> GMSRFWRSFTYFEWRPTPAIHRQLQKIICKYKETFMKQEYTNPYQLVDFDPLFISHLGAPKPLHVSLTRSLLFETEEQRHVFIQ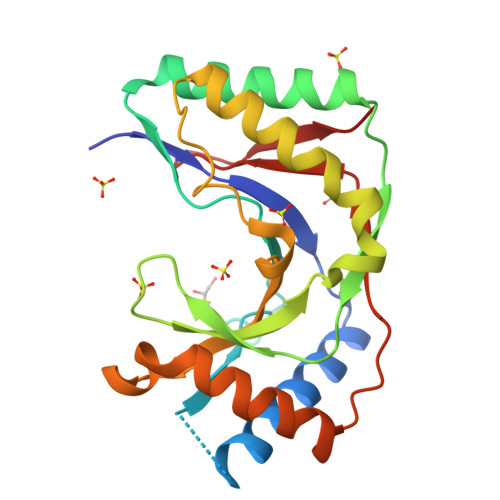EMRNGLRNNEITPFKLQICSYPKLYISERANTLYLGLPVSECPNKAQISPFKTIIAEALQKSGISNYQDLIVSRQNLHVSIAIASNPSKATLKRYQQLNETMGALLLLNNDFAYKLEFLVNSIYCDENRHSIRIPFN>DPAGADAGSAVPFHGAHQAGIATPVQDRLHFAAFDVTTEDRAAFVALLKEWTAAARRLTAGHAVGEGAYGGLPEAPPDDTGEALGLKPSRLTLTIGFGPSLFTRFGLADLRPEALADLPKFPGDNLDRARSGGDLCVQACADDPQVAVHAIRNLARIGFGKVVVRWSQLGFGKTSSTTPDKQTPRNLLGFKDGTRNIAGTEKDRLDRFVWAAEKDGTPWMTGGSYLVARRIRMHIETWDRASLQEQEDVFGRDKGEGAPVGKAKERDEPFLKAMKPDAHVRLAHPDSNGGATLLRRGYSFTDGTDGLGRLDAGLFFLAYQRDIRTGFVPVQRNLATDALNEFIQHVGSAVFAVPPGVRDADDWWGSTLFGKEA[2x]

Here, a highly sample-efficient methodology to measure serial crystallography data from microcrystals by raster scanning within standard in situ 96-well crystallization plates is described. Structures were determined from very small quantities of microcrystal suspension and the results were compared with those from other sample-delivery methods. We demonstrate that raster-scan serial data collection within crystallization plates can be an easily accessible and rapid method of assessing microcrystallization experiments and determining suitable-quality room-temperature structures.

DtpAa crystallized in the monoclinic space group P21, representing a much lower symmetry than was the case for HEWL (P43212) and making it an important test system for the general applicability of this method. This protein was chosen as it has well characterized responses to radiation damage, with real-world serial crystallography studies published using both synchrotron and XFEL data. However, the increase in completeness from eight to 12 drops was about 2%, while it increased by only 0.02% on increasing from 12 to 35 drops. Additionally, the I/σ(I) improved significantly from 12.6 to 19.7 when comparing eight and 12 drops, while it only improved marginally from 19.7 to 21.8 when comparing 12 and 35 drops. Using these statistics as an example, it is clear to see that while adding four additional drops to the initial eight-drop data set led to a large increase in data quality (with an additional 20 min of data collection), the addition of 23 extra drops only led to a marginal increase in comparison, but led to a significantly longer data-collection time (nearly two additional hours of data collection). More amino acids, water molecules and alternate conformations could be convincingly modelled when 35 drops were merged (22 854 merged diffraction patterns), although these were removed for the 12-drop and eight-drop data sets (10 054 and 5360 merged diffraction patterns, respectively) where the electron density was not as clear. Despite the difference in merging statistics, the maps for all three were of similar quality, in particular noting the well defined waters around the heme in chain A in each case. The electron density corresponding to the Fe—OH2 bond is also marginally clearer in the maps from 12 and 35 wells (10 054 and 22 854 merged diffraction patterns, respectively), but this would not hinder map interpretation from the eight-drop data set (5360 merged diffraction patterns) within a screening context.>GPGADRAQDHNNNNTPRNSNYVVEEEEVSEEEEEAIMMPDFGDHVDTSIFGQILEMDEGDDHDFSAPLVLNFFEQAEETFQKMETALNNKDLPELSKLGHFLKGSSATLGFTKIRDSCQLIQQYGHGLNVDGSSEPDEGVCLKKIAEALASAAVDTVALHKMMR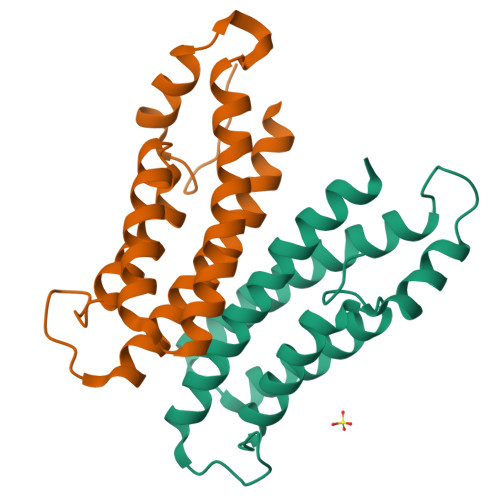EFFEY[2x]>[3x]SNADPSAAVARAFAPLLDQYDVPGMAVAVTVDGRQHFYEFGVVSKQTQAPVTRDTLFEIGSVSKTFTATLAGYAATRGVLNLDDHPGRYLPALAGTPIDRAELRNLGTYTAGGLPLQFPESVTDDEQMIAYFQQFQPVTAPGKIRQYSNPSVGLLGHISARALGGQFTDLMQSQILTGLGLRRSFVDVTDEAMDFYAWGYDKKNHPVRVNPGVFDAEAYGVKSTTADMIRFIEHNIDPGALEPTLREAV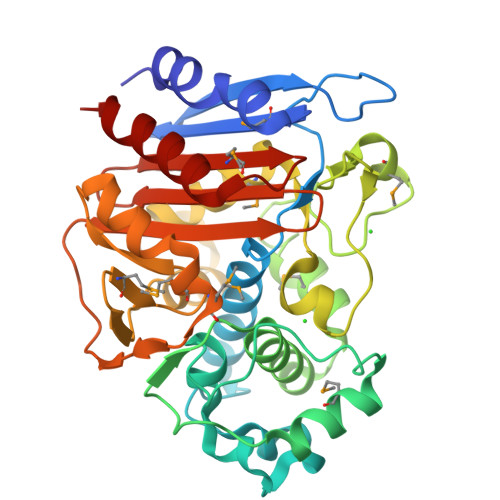KSTQVGYYKVGPMVQDLGWEQYPYPVALDQLLAGNSGEMAMSPQAATAIAPPSVGSALFNKTGSTDGFGAYAAFVPERRIGIVMLANKNFPIPARVTAAHTVLDALDA9-(3,5-dichloro-4-hydroxyphenyl)-1-{trans-4-[(dimethylamino)methyl]cyclohexyl}-3-methyl-3,4-dihydropyrimido[5,4-c][1,5]naphthyridin-2(1H)-one 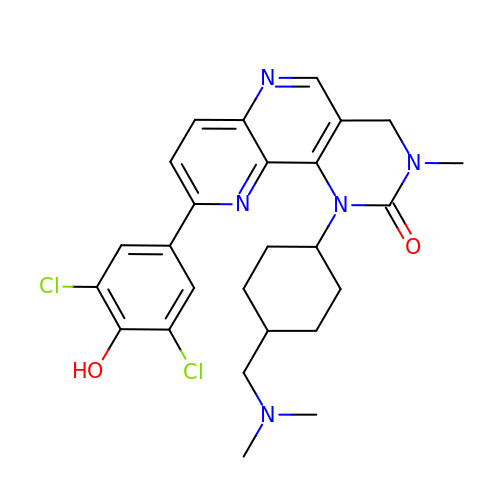| C26 H29 Cl2 N5 O2 | HHDFQGMZNYJMHI-RZDIXWSQSA-N6-CHLORO-N-[(3S)-1-[(1S)-1-DIMETHYLAMINO-2,3-DIHYDRO-1H-INDEN-5-YL]-2-OXO-PYRROLIDIN-3-YL]NAPHTHALENE-2-SULFONAMIDE 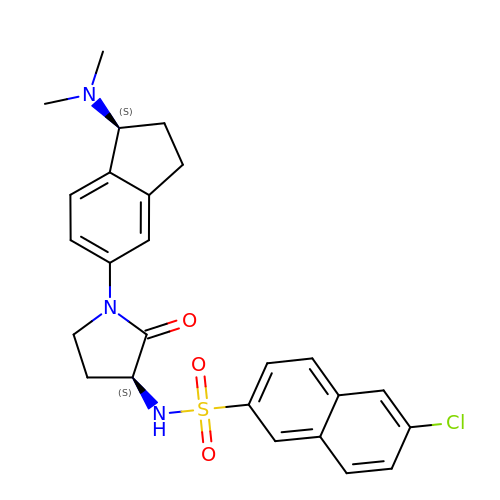| C25 H26 Cl N3 O3 S | DBFTVRMJVISJEX-ZEQRLZLVSA-N6-[([1,1'-biphenyl]-4-yl)ethynyl]-9-beta-D-ribofuranosyl-9H-purine | C24 H20 N4 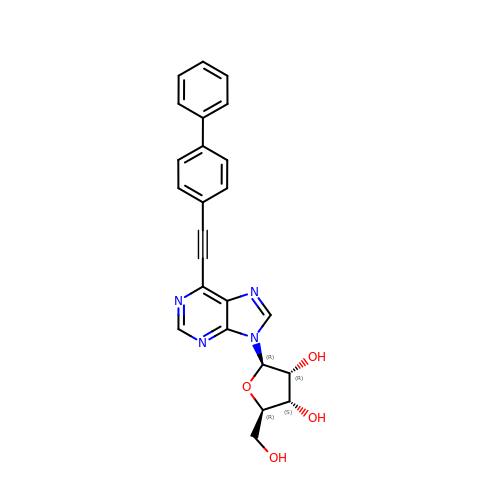O4 | VJQTZOVBQVSIJJ-VDEHWKIFSA-N> MPRKAREYPEEGEFVVATVKRIHNYGAFLELDEYPGKEAFMHISEVASTWVRNIRDYLKEGQKVVAKVIRVDPRKGHIDLSLRRVTQQQRKAKLQEFKRAQKAENLLRLAAEKLGKDFEAAWREVWVPLEEEWGEVYAAFEDAAKDGIEVLKGHVPDEWLPVLKEIVENYVEVPTVTIDAEFEITVPKPNGVEIIKEALIRARDRANKEKDIEVKFTYQGAPRYRIDITAPDYYKAEEVLEDIAEEILRVIKQAGGEATLLRKEKRIRKVKKRKK;> MGEEFEKLMKKFENVNKDGEIVEDEDEWEEFFKQEEYVKIPKDRIAVLIGKKGQTKKEIEKRTKTKITIDSETGEVWITSTKETEDPLAVWKARDIVLAIGRGFSPERAFRLLNEGEYLEIINLTDIIIGNEKNALPRVRGRIIGRKGRTRQIIE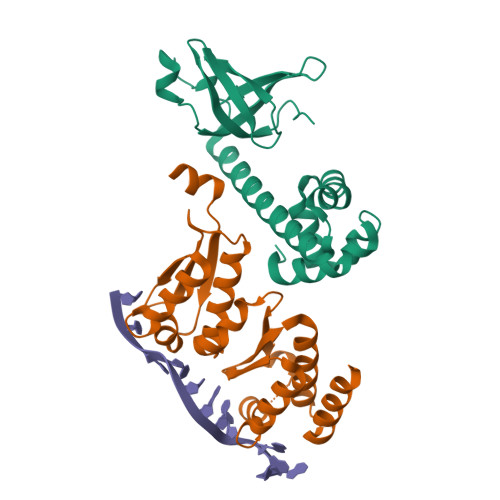EMSGASVSVYGKTVAIIGNPIQIEIAKTAIEKLARGSPHGSVYRYLERRKKDLELEGAMYYENL> MKKEKIDLFYGALLHDIGKVIQRATGERKKHALVGADWFDEIADNQVISDQIRYHMANYQSDKLGNDHLAYITYIADNIASGVDRRQSNEESDEDASAKIWDTYTNQADIFNVFGAQTDKRYFKPTVLNLKSKPNFASATYEPFSKGDYAAIATRIKNELAEFEFNQAQIDSLLNLFEAILSFVPSSTNSKEIADISLAEHSRLTAAFALAIYDYLEDKGRH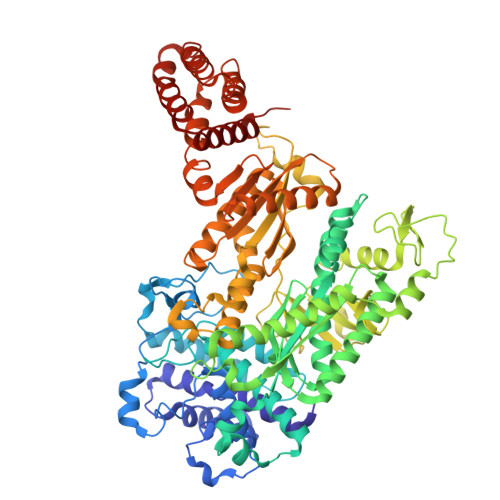NYKEDLFTKASAFYEEEAFLLASFDLSGIQDFIYNIATSGAAKQLKARSLYLDFMSEYIADSLLDKLGLNRANLLYVGGGHAYFVLANTEKTVETLVQFEKDFNQFLLANFQTRLYVAFGWGSFAAKDIMSELNSPESYRQIYQKASRMISEKKISRYDYRTLMLLNRGGKSSERECEICHSVENLVSYHDQKVCDICRGLYQFSKEIAHDHFIITENEGLPIGPNACLKGVAFEKLSQESFSRVYVKNDYKAGTIKATHVFVGDYQCDEIHKYAALSKNEDGLGIKRLAVVRLDVDDLGAAFMAGFSRQGNGQYSTLSRSATFSRSMSLFFKVYINQFASDKKLSIIYAGGDDVFAIGSWQDIIAFTVELRQNFIKWTNGKLTLSAGIGLFADKTPISLMAHQTGELEEAAKGNEKDSISLFSSDYTFKFDRFITNVYDDKLEQIRYFFNHQDERGKNFIYKLIELLRNYESEEKMNVARLAYYLTRLEELTDKDERDKFKQFKKLFFKWYTNNESDRKEAELALLLYVYEIRKD>[2x]MKKTKIVCTIGPKTESEEMLAKMLDAGMNVMRLNFSHGDYAEHGQRIQNLRNVMSKTGKTAAILLDTKGPEIRTMKLEGGNDVSLKAGQTFTFTTDKSVIGNSEMVAVTYEGFTTDLSVGNTVLVDDGLIGMEVTAIEGNKVICKVLNNGDLGENKGVNLPGVSIALPALAEKDKQDLIFGCEQGVDFVAASFIRK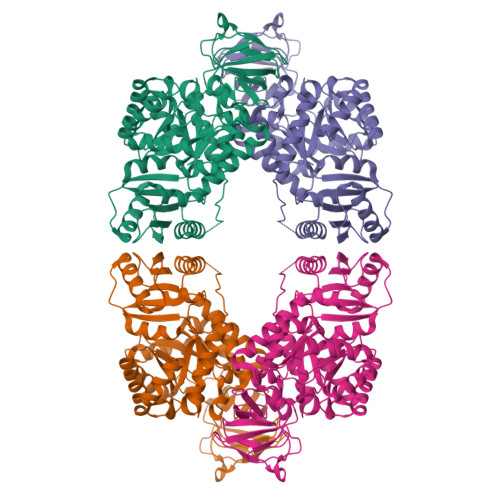RSDVIEIREHLKAHGGENIHIISKIENQEGLNNFDEILEASDGIMVARGDLGVEIPVEEVIFAQKMMIEKCIRARKVVITATQMLDSMIKNPRPTRAEAGDVANAILDGTDAVMLSGESAKGKYPLEAVSIMATICERTDRVMNSRLEFNNDNRKLRITEAVCRGAVETAEKLDAPLIVVATQGGKSARAVRKYFPDATILALTTNEKTAHQLVLSKGVVPQLVKEITSTDDFYRLGKELALQSGLAHKGDVVVMVSGALVPSGTINTASVHVL> MSLPLLRPFETVSLENAVEDLVVRFILNVPPEDLSTVERVLFHFEEASWFYTDFVKLMNPYLPNLSIKSFSKIVIDICPLIWNWDITPENALVKFSNYKKTIPVRGAAIFNDSLSKILLLRGINSKHWSFPRGKIGKDEDDVACCIREVKEETGFDLTGFIDADQYVERNMNGKNFKIFLVKGVPEDFEFKPEHKNEIQAIEWKDFKKLSKAITKNEGSAKVFLVNSMIRPLSLYVKNEKRAKDENKLK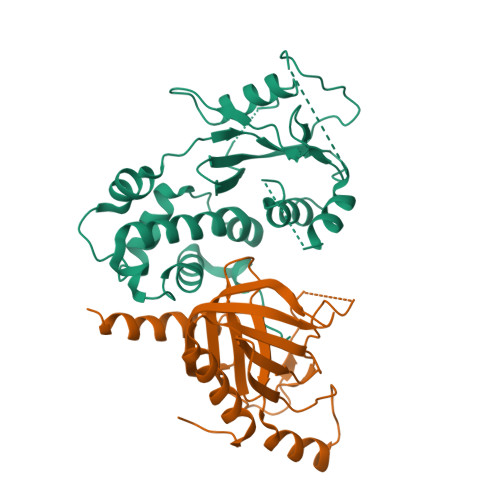LYAEEHLKSILGLNKKENKIVLDAGRHHHHHH;> MSTETLEIYRKALNFNVIARYDPKIKQLLFHTPHATVYKWGDDNWNKLEYQGVLAIYLRDVGDKEAILPEVSSYDDTITGQQSEANTPHVLTGHDIYNYGLIIMNRINPDNFSLAIAPNSVLNKRKLFAPNREEELEPMKVEVRDDLVMIKTLKKEVYGIWVHTPEDRQNIYELIKYLLENEPTDSFT> MKTVTVKNLIIGEGMPKIIVSLMGRDINSVKAEALAYREATFDILEWRVDHFMDIASTQSVLTAARVIRDAMPDIPLLFTFRSAKEGGEQTITTQHYLTLNRAAIDSGLVDMIDLELFTGDADVKATVDYAHAHNVYVVMSNHDFHQTPSAEEMVLRLRKMQALGADIPKIAVMPQSKHDVLTLLTATLEMQQ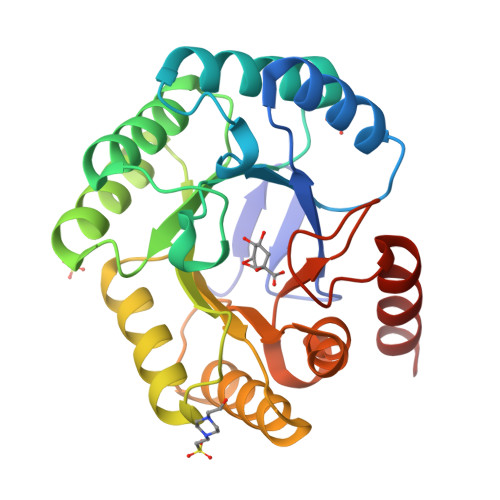HYADRPVITMSMAKEGVISRLAGEVFGSAATFGAVKQASAPGQIAVNDLRSVLMILHNA>MSGDNGMTEEKLRRYLKRTVTELDSVTARLREVEHRAGEPIAIVGMACRFPGDVDSPESFWEFVSGGGDAIAEAPADRGWEPDPDARLGGMLAAAGDFDAGFFGISPREALAMDPQQRIMLEISWEALERAGHDPVSLRGSATGVFTGVGTVDYGPRPDEAPDEVLGYVGTGTASSVASGRVAYCLGLEGPAMTVDTACSSGLTALHLAMESLRRDECGLALAGGVTVMSSPGAFTEFRSQGGLAADGRCKPFSKAADGFGLAEGAGVLVLQRLSAARREGRPVLAVLRGSAVNQDGASNGLTAPSGPAQQRVIRRALENAGVRAGDVDYVEAHGTGTRLGDPIEVHALLSTYGAERDPDDPLWIGSVKSNIGHTQAAAGVAGVMKAVLALRHGEMPRTLHFDEPSPQIEWDLGAVSVVSQARSWPAGERPRRAGVSSFGISGTNAHVIVEEAPEADEPEPAPDSGPVPLVLSGRDEQAMRAQAGRLADHLAREPRNSLRDTGFTLATRRSAWEHRAVVVGDRDEALAGLRAVADGRIADRTATGQARTRRGVAMVFPGQGAQWQGMARDLLRESQVFADSIRDCERALAPHVDWSLTDLLSGARPLDRVDVVQPALFAVMVSLAALWRSHGVEPAAVVGHSQGEIAAAHVAGALTLEDAAKLVAVRSRVLRRLGGQGGMASFGLGTEQAAERIGRFAGALSIASVNGPRSVVVAGESGPLDELIAECEAEAHKARRIPVDYASHSPQVESLREELLTELAGISPVSADVALYSTTTGQPIDTATMDTAYWYANL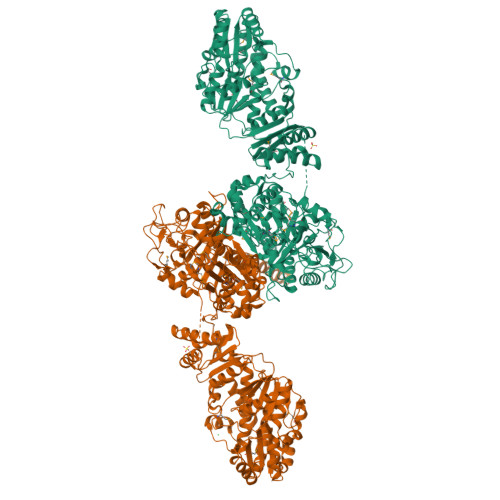REQVRFQDATRQLAEAGFDAFVEVSPHPVLTVGIEATLDSALPADAGACVVGTLRRDRGGLADFHTALGEAYAQGVEVDWSPAFADARPVELPVYPFQRQRYWLPIPTGGRARDEDDDWRYQ[6x]> MVSLPRMVYPQPKVLTPCRKDVL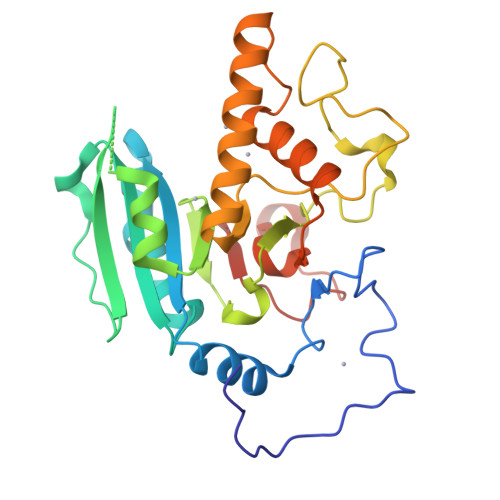VVTPWLAPIVWEGTFNIDILNEQFRLQNTTIGLTVFAIKKYVAFLKLFLETAEKHFMVGHRVHYYVFTDQPAAVPRVTLGTGRQLSVLEVRAYKRWQDVSMRRMEMISDFCERRFLSEVDYLVCVDVDMEFRDHVGVEILTPLFGTLHPGFYGSSREAFTYERRPQSQAYIPKDEGDFYYLGGFFGGSVQEVQRLTRACHQAMMVDQANGIEAVWHDESHLNKYLLRHKPTKVLSPEYLWDQQLLGWPAVLRKLRFTAVPKNHQAVRNP1-(2-deoxy-2-methyl-beta-D-arabinofuranosyl)-5-ethynylpyrimidine-2,4(1H,3H)-dione | C12 H14 N2 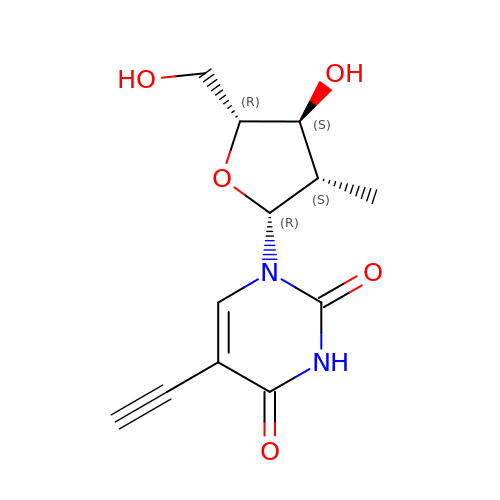O5 | HBALXYGFMJGYHQ-GTQWGBSQSA-N Enzymes of the vanillyl alcohol oxidase/p-cresol methyl hydroxylase (VAO/PCMH) superfamily are found across all kingdoms where they perform a range of metabolic functions. These flavoproteins share a conserved FAD-binding domain and a more variable substrate-binding domain that enables interactions with a range of substrates. One of these, the 4-phenol oxidases/dehydrogenases, catalyzes the oxidation of para-substituted phenolic compounds. A fundamental distinction is that the oxidases efficiently react with oxygen producing hydrogen peroxide whereas the dehydrogenases hardly react with oxygen and typically employ other proteins, such as cytochrome c, as acceptors.

We further studied the P151G mutation to assess the effect of removing en bloc the side chain, and P151N and P151T to test the introduction of hydrogen-bonding groups. The P151G mutation was found to elicit the same oxidase-activating effect of P151L whereas P151T and P151N conserve the properties of a dehydrogenase. Spectrophotometric measurements confirmed that the vanillyl alcohol-reduced P151N and P151T proteins are hardly re-oxidized by molecular oxygen though they retain dehydrogenase activity while P151G can effectively turn over using oxygen as co-substrate and the product is formed. Conversely, in the dehydrogenase variants (P151N and P151T), like in the wild-type structure, the loop obstructs the access to the N5 atom. Conversely, no tunnels are present in the wild type and the dehydrogenase mutants where the flavin re face remains fully shielded by residue 151 and Trp153.

>[3x]MAAPLPEGVSAEAMSSALDRFARIVGADWVFTEDKITPYEDPYTISNDETEHRPYAAVAPASTEEVQEIVRVANEFGVPLWPVSRGKNFAYGGAAPVMSGTVVLDMNRMNRILEVNEEFGYALVEPGVSYFELYDYIQEKGLKLWIDVPDNGWGSVVGNALDHGIGYTPYGDHFAMQCGMEVVLPNGEVVRTGMGAMPGNNTWQLFKYGYGPYVDGIFSQSNFGVVTKMGIWLMPEPAGYRPYLITFENEDDIETVTERLRPLKVAGVIQNGATVRSLVLDAAITRTKSQYYDGDGPIPPSVAKTMMADLDLGMWNFCGALYGPPPVMDTLWTAIRDSFADIPGVKFYFPEDRRHKVDLLLHRAETMKGVPKLTEFNFLNWDGGGGHVGFSPVSPITGKDAIKQYNMVSSRVREYGFDYMGLLAIGWRDLHHVTVIVYDKTDPDERKKLDELFNILVDEAAAEGYGEYRTHIRYMDRIAKTYSWNDNALWKMHETIKDALDPNGILAPGKSGIWGKNRRKA~{N}-[3,5-bis[[4-[(4-bromophenyl)methyl]piperazin-1-yl]methyl]phenyl]-2-ethyl-2-methanoyl-butanamide 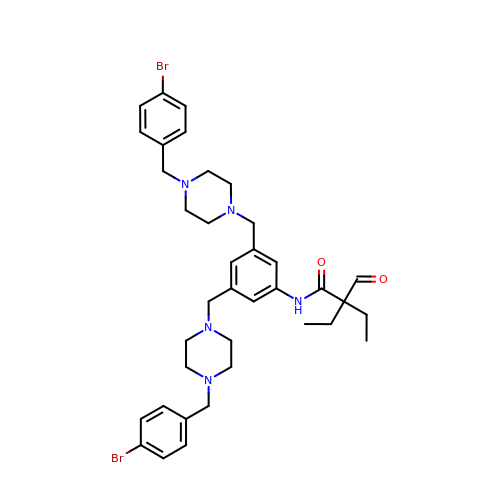| C37 H47 Br2 N5 O2 | FVBNIXZASNLFMF-UHFFFAOYSA-N> MADYDKYFSNVQINNLSYGVYTSGGKE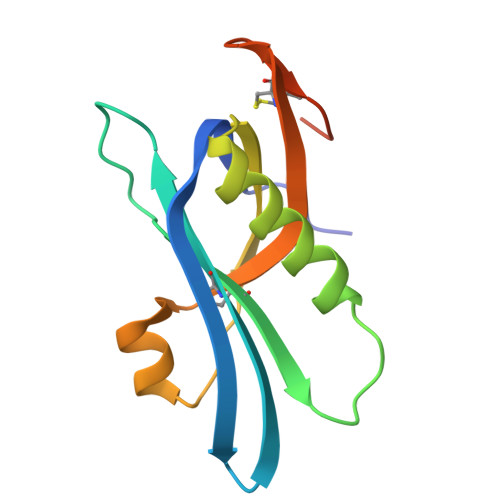SQFFCIGIKRDNVTLPIHNMCKVDVFGSHKQGFDAMMEMAKYYYATGESIRVYYKENVWSDSEFKKAFSTNELISLSTCSSSDYCMGPQKDTLEHHHHHH> ARHFVLNTGAKIPSVGLGSWQSDPGVVGNAVYAAVKAGYRHIDCARVYGNEKEIGLALKKLFEEGVVKREDMFITSKLWNDHHAPEDVPEALNDSLNDLQLEYLDLYLIHWPFRVKKGTNTSPENFVTPDFPATWGAMEKLYDAGKARAIGVSNFSSKKLGDLLAVARVPPAVDQVECHPGWQQTKLHSFCQSTGVHLTAYSPLGSPGTTWMNGNVLKEPIIISIAEKLGKTSAQVALRWNIQMGHSVLPKS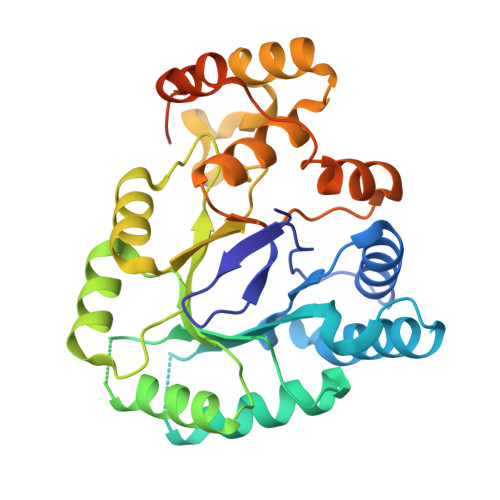TNEERIKQNLDVYDWSIPDDLLAKFSEIKQARLLRGNFIVNPESVYKTHEELWDGEL>GMTRIASHRGGTLEFGDSTPHGFTATAAMALEEVEFDLHPTADGAIVVHHDPTLDATTDMTGAIVDMTLAKVKTATIRYGAGSHPMTLEELCALYVDSHVNFRCEIKPGVDGLPYEGFVALVIAGLERHSMLERTTFSSFLLASMDELWKATTRPRLWLVSPSVLQQLGPGAVIETAIAHSIHEIGVHIDTADAG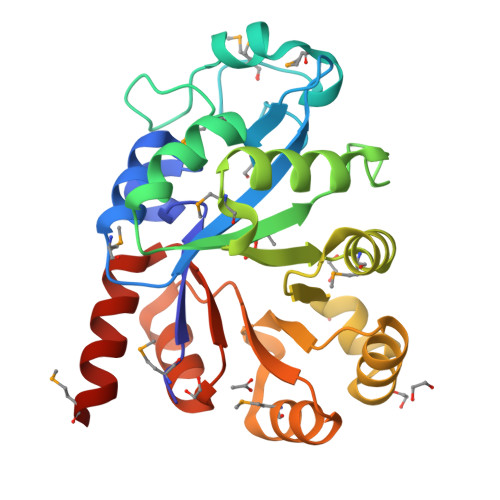LMAQVQAAGLDFGCWAAHTPSQITKALDLGVKVFTTDRPTLAIALRTEHRMEASV[2x]> MSGGVSPVEQVAAGDMDDTAARFCVQKHSWDGLRNIIHGSRKSSGLIVSKAPHDFQFVQKPDESGPHSHRLYYLGMPYGSRENSLLYSEIPKKVRKEALLLLSWKQMLDHFQATPHHGVYSREEELLRERKRLGVFGITSYDFHSESGLFLFQASNSLFHCRDGGKNGFMVSPMKPLEIKTQCSGPRMDPKICPADPAFFSFINNNDLWVANIETGEERRLTFCHQGSASVLDNPKSAGVATFVIQEEFDRFTGCWWCPTASWEGSGGLKTLRILYEEVDESEVEVIHVPSPALEERKTDSYRYPRTGSKNPKIALKLAELQTDHQGKIVSSCEKELVQPFSSLFPKVEYIARAGWTRDGRYAWAMFLDRPQQRLQLVLLPPALFIPTLESEAQWQEAARAIPKNVQPFIIYEEVTNVWINVHDIFHPFPQAEGQQDFCFLRANECKTGFCHLYRVTVDLKTNDYDWTEPLSPAEDEFKCPIKEEVALTSGEWEVLSRHGSKIWVNEQTKLVYFQGTKDTPLEHHLYVVSYESAGEIVRLTTPGFSHSCSMSQNFDMFVSHYSSVSTPPCVHVYKLSGPDDDPLHKQPRFWASMMEAASCPPDYVPPEIFHFHTRADVQLYGMIYKPHTLQPGRKHPTVLFVYGGPQVQLVNNSFKGIKYLRLNTLASLGYAVVVIDGRGSCQRGLHFEGALKNQMGQVEIEDQVEGLQYVAEKYGFIDLSRVAIHGWSYGGFLSLMGLIHKPQVFKVAIAGAPVTVWMAYDTGYTERYMDVPENNQQGYEAGSVALHVEKLPNEPNRLLILHGFLDENVHFFHTNFLVSQLIRAGKPYQLQIYPNERHSIRCRESGEHYEVTLLHFL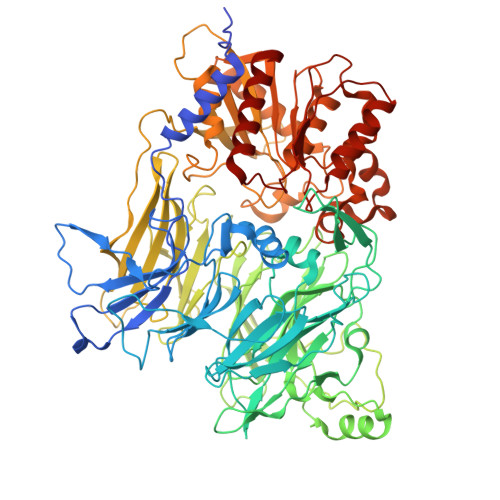QEHL>MSELALIQKAIEESQQKMTQLFDAQKAEIESTGQVSKQLQSDLMKVQEELTKSGTRLFDLEQKLASGAENPGEKKSFSERAAEELIKSWDGKQGTFGAKTFNKSLGSDADSAGSLIQPMQIPGIIMPGLRRLTIRDLLAQGRTSSNALEYVREEVFTNNADVVAEKALKPESDITFSKQTANVKTIAHWVQASRQVMDDAPMLQSYINNRLMYGLALKEEGQLLNGDGTGD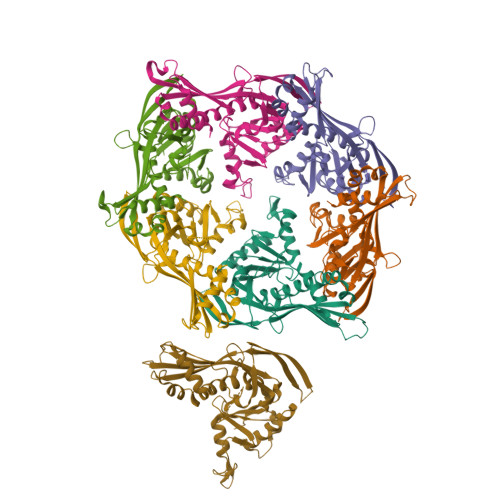NLEGLNKVATAYDTSLNATGDTRADIIAHAIYQVTESEFSASGIVLNPRDWHNIALLKDNEGRYIFGGPQAFTSNIMWGLPVVPTKAQAAGTFTVGGFDMASQVWDRMDATVEVSREDRDNFVKNMLTILCEERLALAHYRPTAIIKGTFSSGS[7x]>MGSITENTSWNKEFSAEAVNGVFVLCKSSSKSCATNDLARASKEYLPASTFKIPNAIIGLETGVIKNEHQVFKWDGKPRAMKQWERDLTLRGAIQVSAVPVFQQIAREVGEVRMQKYLKKFSYGNQNISGGIDKFWLEGQLRISAVNQVEFLESLYLNKLSASKENQLIVKEALVTEAAPEYLVHSKTGFSGVGTESNPGVAWWVGWVEKETEVYFFAFNMDIDNE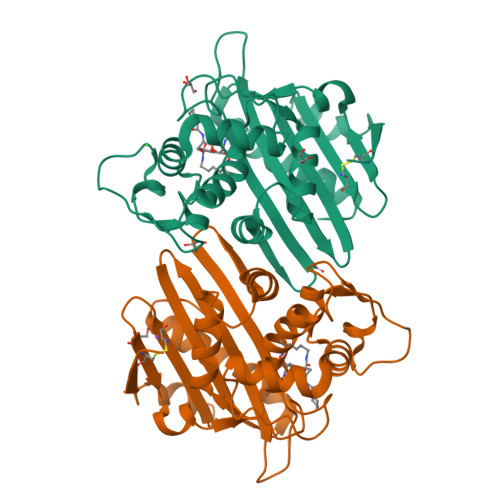SKLPLRKSIPTKIMESEGIIGG[2x]P. aeruginosa encodes three distinct T6SS hemolysin coregulated protein (Hcp) secretion islands (named H1-to H3-T6SS) that act against both prokaryotic and eukaryotic cells. TplE, a novel H2-T6SS-dependent lipase effector, was recently identified. TplE is an antibacterial lipolytic toxin and TplEi interacts with TplE to provide protection from TplE. TplE, a new T6SS trans-kingdom toxin, targets the conserved and essential cell membranes of rival bacteria to cause bacteriolysis, while TplEi functions as a cognate immunity protein to prevent self-intoxication.

Next, we also obtained crystals of TplEi alone and determined the structure at 3.06 Å resolution using SAD. The structure of TplEi alone is very similar to that observed in the peptide-bound form, with only a handful of side chains with different rotamer conformations. Specifically, the side chains of residues such as Mse274 move out to avoid clashes, F230 and R209 are closer to the peptide, and residues E219, E211, and K266 change their side chain conformations to form hydrogen bonds or salt bridges with the peptide. The similarity between the free and peptide-bound forms suggests that the TplEi structure is highly compact and rigid, and the “L” peptide binds via a structurally stable pocket on TplEi. TplEi is assembled into a highly rigid structure, not only in the apo but also in the peptide-bound structure.

>MGSSHHHHHHSSGLVPRGSHMSSSRSSSMDKTGWITHCFGRFLIDLPPDAVINAGYYLWGDRIEYLDDKPTELAARVDRLEQEWRTQRHKSKGNMFLRKIDFGNESVGLLSWSSEVASKTYLLDTYVTSKPTWHVYRWKGKVSVDREQHAVEISRALARNLRSRAPKEIPSEPGFCIDHAYIAGDSFQVERFGVGVTFPEHPGARFEFRSSTGAELNSLLERVDGFVQNMLSTFAGMETLRKGKHPVGSLPGEEYLVAGSDKGQRGYTFMWEVQGKEESLTEPNLTAGLAVLERSNENGKPPPPAFKSDKEALELWDTIVDSIRVRPTSSSPRGGNAGPSPAPKPATPGGQTLGDHYVYEEFLSSLKPKDSWLDDL[2x]> MVGLIWAQATSGVIGRGGDIPWRLPEDQAHFREITMGHTIVMGRRTWDSLPAKVRPLPGRRNVVLSRQADFMASG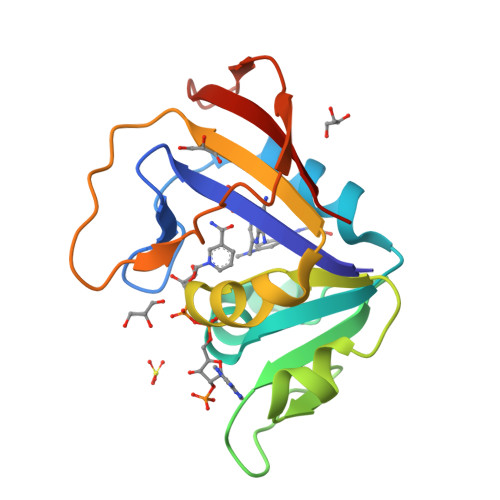AEVVGSLEEALTSPETWVIGGGQVYALALPYATRCEVTEVDIGLPREAGDALAPVLDETWRGETGEWRFSRSGLRYRLYSYHRS>MESANDKELDQLLNEHFAGRVVRKDLTKLIKEGANVPVYVLEYLLGMYCASDDPEIIEQGLRNVKTVLAENYVRPDEAEKVKSLVRERGSYKVIDRVTVKLNERKDKYEASFSNLGIKDAEISAGIVKEYEKLLVGGIWVIATLSYYFEEGQTSSPFGVSLLKPIQMPNMNMDELFSGRAALSTDQWRESLIRSIGMEPASLKEDVQWHLLARMVPFVENNYNVCELGPRGTGKSHIYKECSPNSILVSGGQTTVANLFYNMSSRRIGLVGLWDVVAFDQVAGISFKDKDGVQIMKDYMASGSFARGREQMEASASMVFVGNINQSVESLVKTSHLLAPFPEAMIDSAFFDRFHAYIPGWEIPKMRPEFFTNRYGLIVDYLAEFFREMRKRSFADSIEKYFKLGNNLNQRDVIAVRKTVSGLMKLLYPHGQFNKEDVRQCLEYALQVRRRVKEQLKKIGGMEFYDVHFSYIDNDTLEEHFVSVKEQGGGGLIPEGPAKPGFLYTIGLSNKGMPGLYRLELQVTKGSGKLATSGLWNSSSAKEQVKIAFDYFKANASRISGGSKVMEH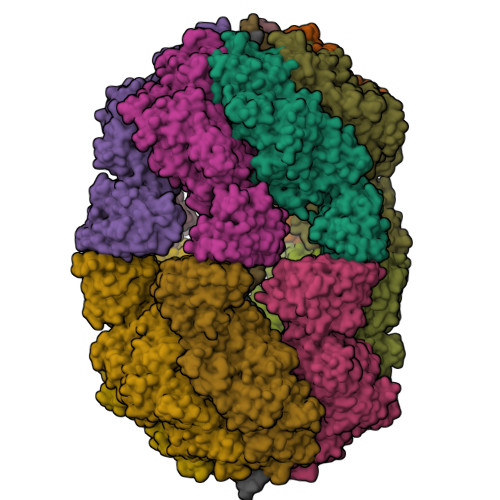DFHLHVVELQNTGPLSHLALPSLVAFASGLLGRSVQSQMVVLGDMSLGGSVTPVESIAECLQVAFDAGAKKVALPMSSAADIPTIPVELFTKFQTSFYADPVDAVFKGLGVD[12x]Acarviosin | C14 H25 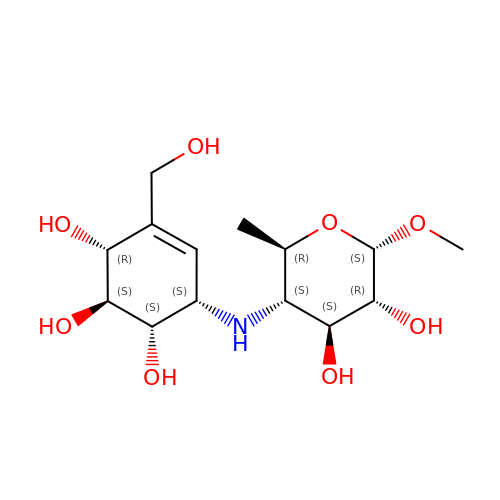N O8 | KFHKERRGDZTZQJ-SHCNSHNESA-N HP0935 is a small (161 amino acids long) single GNAT domain-containing protein belonging to type IV protein acetyltransferases. A biochemical study showed that HP0935, the only known protein acetyltransferase in H. pylori, can acetylate free lysine amino acid and lysine residues in proteins. The crystal structure of HP0935 revealed a conserved GNAT fold, characteristic of the GNAT superfamily. The structure of HP0935 is composed of seven β-strands and four α-helices arranged in a topology—β1· α1· α2· β2· β3· β4· α3· β5· α4· β6· β7.

To gain structural insights, the crystal structures of HP0935 in its apo and ACO-bound forms were determined to be 2.00 Å and 2.40 Å resolution, respectively (see Experimental procedures). ACO is bound in a tunnel formed by the α1-α2 loop, β4, β4-α3 loop, α3, β5, β5-α4 loop, and α4. While the ACO is bound in a bent (L-shaped) conformation, the pyrophospha forms hydrogen bonds with residute moiety is accommodated by the P-loop, and the pantotheine moietyes on the β4 side of the wedge-shaped cleft (residues F81 and I83), mimicking the hydrogen bonding pattern of a parallel β-sheet structure. The adenine moiety of ACO is stabilized by hydrogen bonding with side chains of residues S89 and N125. The carbonyl oxygen of ACO’s acetyl group forms a hydrogen bond with the backbone amide (NH) of the β-bulge residue F81, which may stabilize the tetrahedral intermediate during the acetylation reaction. The apo- and ACO-bound HP0935 crystallized in distinct space groups, C2 and P61, respectively. In contrast, these regions were well-ordered in the ACO-HP0935 structure, with a significant conformational change in the α1-α2 loop. In contrast, in ACO-HP0935, the loop shifts toward ACO, adopting a proximal conformation. Despite a low overall Cα RMSD between the two structures (1.95 Å), the α1-α2 loop displayed high residue-wise RMSD values, with residues N25 and F29 shifting towards ACO, by 6.00 Å and 9.44 Å, respectively. This transition constricts the ACO-binding cleft, likely stabilizing ACO and facilitating acetyl transfer. In contrast, in the proximal conformation, the loop is fully ordered and stabilized by interactions with the β6-β7 hairpin and symmetry-related molecules.

>SMVTIKVFSPKYPTELEEFYAERIADNPLGFIQRLDLLPSISGFVQKLREHGGEFFEMREGNKLIGICGLNPINQTEAELCKFHINSAYQSQGLGQKLYESVEKYAFIKGYTKISLHVSKSQIKACNLYQKLGFVHIKEEDCVVELGEETLIFPTLFMEKILS[4x]> MELQPPEASIAVVSIPRQLPGSHSEAGVQGLSAGDDSETGSDCVTQAGLQLLASSDPPALASKNAEVTVETGFHHVSQADIEFLTSIDPTASASGSAGITGTMSQDTEVDMKEVELNELEPEKQPMNAASGAAMSLAGAEKNGLVKIKVAEDEAEAAAAAKFTGLSKEELLKVAGSPGWVRTRWALLLLFWLGWLGMLAGAVVIIVRAPRCRELPAQKWWHTGALYRIGDLQAFQGHGAGNLAGLKGRLDYLSSLKVKGLVLGPIHKNQKDDVAQTDLLQIDPNFGSKEDFDSLLQSAKKKSIRVILDLTPNYRGENSWFSTQVDTVATKVKDALEFWLQAGVDGFQVRDIENLKDASSFLAEWQNITKGFSEDRLLIAGTNSSDLQQILSLLESNKDLLLTSSYLSDSGSTGEHTKSLVTQYLNATGNRWCSWSLSQARLLTSFLPAQLLRLYQLMLFTLPGTPVFSYGDEIGLDAAALPGQPMEAPVMLWDESSFPDIPGAVSANMTVKGQSEDPGSLLSLFRRLSDQRSKERSLLHGDFHAFSAGPGLFSYIRHWDQNERFLVVLNFGDVGLSAGLQASDLPASASLPAKADLLLSTQPGREEGSPLELERLKLEPHEGLLLRFPYAA;> MAGHTQQPSGRGNPRPAPSPSPVPGTVPGASERVALKKEIGLLSACTIIIGNIIGSGIFISPKGVLEHSGSVGLALFVWVLGGGVTALGSLCYAELGVAIPKSGGDYAYVTEIFGGLAGFLLLWSAVLIMYPTSLAVISMTFSNYVLQPVFPNCIPPTTASRVLSMACLMLLTWVNSSSVRWATRIQDMFTGGKLLALSLIIGVGLLQIFQGHFEELRPSNAFAFWMTPSVGHLALAFLQGSFAFSGWNFLNYVTEEMVDARKNLPRAIFISIPLVTFVYTFTNIAYFTAMSPQELLSSNAVAVTFGEKLLGYFSWVMPVSVALSTFGGINGYLFTYSRLCFSGAREGHLPSLLAMIHVRHCTPIPALLVCCGATAVIMLVGDTYTLINYVSFINYLCYGVTILGLLLLRWRRPALHRPIKVNLLIPVAYLVFWAFLLVFSFISEPMVCGVGVIIILTGVPIFFLGVFWRSKPKCVHRLTESMTHWGQELCFVVYPQDAPEEEENGPCPPSLLPATDKPSKPQ

The Alanine-Serine-Cysteine transporter 1 (Asc-1 or SLC7A10) forms a crucial heterodimeric transporter complex with 4F2hc (SLC3A2) through a covalent disulfide bridge. This complex enables the sodium-independent transport of small neutral amino acids, including L-Alanine (L-Ala), Glycine (Gly), and D-Serine (D-Ser), within the central nervous system (CNS). Here, we present cryo-electron microscopy (cryo-EM) structures of the human Asc-1-4F2hc complex in its apo state, D-Ser bound state, and L-Ala bound state, resolved at 3.6 Å, 3.5 Å, and 3.4 Å, respectively. The HAT-specific disulfide bond is found between Cys154 of Asc-1 and Cys211 of 4F2hc.

Overall, both the apo and D-Ser-incubated structures exhibit an inward open conformation, with 12 transmembrane (TM) helices forming the characteristic LeuT-fold. Nevertheless, upon closer examination of the interaction mechanism, significant differences emerge. Apart from the conserved disulfide bond, Asn153 and Gln294 of Asc-1 could form hydrogen bonds with Arg535 and Lys533 of 4F2hc, respectively, in the apo state (inward open Fig. 2b). In the absence of substrate binding, the transporter adopts an inward-facing conformation. When aligning the D-Ser bound structure with the apo state in Asc-1, only a slight movement of TM1a towards the interior is observed. However, upon further comparison between the D-Ser and L-Ala bound structures, or apo and L-Ala bound structures, significant movements are evident in TM1, TM6, and TM8.>[2x]MLKIIRAGMYTTVQDGGRHGFRQSGISHCGALDMPALRIANLLVGNDANAPALEITLGQLTVEFETDGWFALTGAGCEARLDDNAVWTGWRLPMKAGQRLTLKRPQHGMRSYLAVAGGIDVPPVMGSCSTDLKVGIGGLEGRLLKDGDRLPIGKSKRDSMEAQGVKQLLWGNRIRALPGPEYHEFDRASQDAFWRSPWQLSSQSNRMGYRLQGQILKRTTDRELLSHGLLPGVVQVPHNGQPIVLMNDAQTTGGYPRIACIIEADMYHLAQIPLGQPI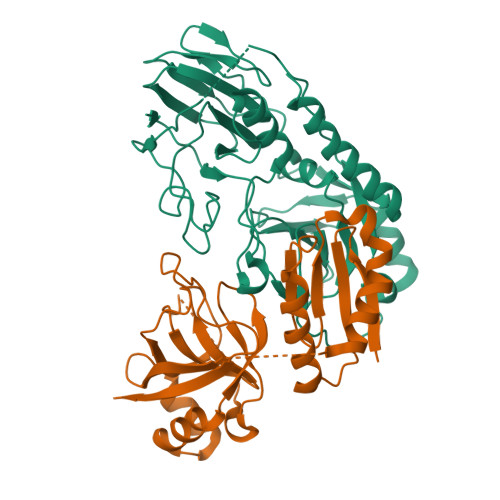HFVQCSLEEALKARQDQQRYFEQLAWRLHNEN;>[2x]MQRARCYLIGETAVVLELEPPVTLASQKRIWRLAQRLVDMPNVVEAIPGMNNITVILRNPESLALDAIERLQRWWEESEALEPESRFIEIPVVYGGAGGPDLAVVAAHCGLSEKQVVELHSSVEYVVWFLGFQPGFPYLGSLPEQLHTPRRAEPRLLVPAGSVGIGGPQTGVYPLATPGGWQLIGHTSLSLFDPARDEPILLRPGDSVRFVPQKEGVC>[4x]MSLFKIRMPETVAEGTRLALRAFSLVVAVDERGGIGDGRSIPWNVPEDMKFFRDVTTKLRGKNVKPSPAKRNAVVMGRKTWDSIPPKFRPLPGRLNVV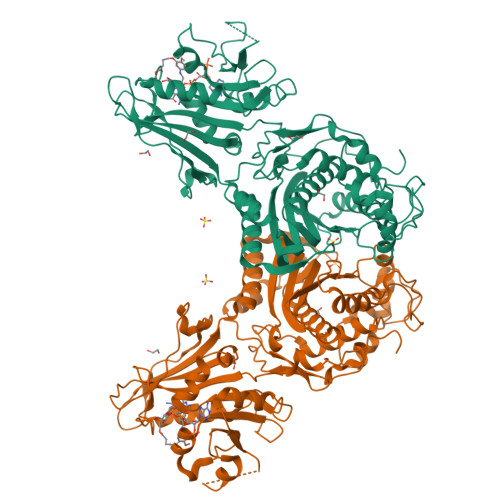LSSTLTTQHLLDGLPDEEKRNLHADSIVAVNGGLEQALQLLASPNYTPSIETVYCIGGGSVYAEALRPPCVHLLQAIYRTTIRASESSCSVFFRVPESGTEAAAGIEWQRETISEELTSANGNETKYYFEKLIPRNREEEQYLSLVDRIIREGNVKHDRTGVGTLSIFGAQMRFSLRNNRLPLLTTKRVFWRGVCEELLWFLRGETYAKKLSDKGVHIWDDNGSRAFLDSRGLTEYEEMDLGPVYGFQWRHFGAAYTHHDANYDGQGVDQIKAIVETLKTNPDDRRMLFTAWNPSALPRMALPPCHLLAQFYVSNGELSCMLYQRSCDMGLGVPFNIASYALLTILIAKATGLRPGELVHTLGDAHVYSNHVEPCNEQLKRVPRAFPYLVFRREREFLEDYEEGDMEVIDYAPYPPISMKMAV> SMGGSPAGQKCFSRTVLAPGVVLIVQQGDLARLPVDVVVNASNEDLKHYGGLAAALSKAAGPELQADCDQIVKREGRLLPGNATISKAGK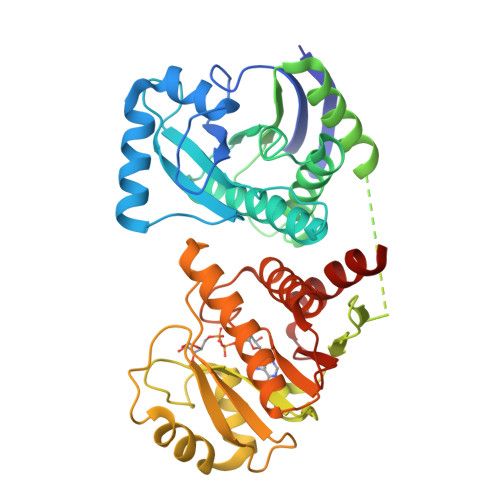LPYHHVIHAVGPRWSGYEAPRCVYLLRRAVQLSLCLAEKYKYRSIAIPAISSGVFGFPLGRCVETIVSAIKENFQFKKDGHCLKEIYLVDVSEKTVEAFAEAVKTVFKATLPDTAAPPGLPPAAAGPGKTSWEKGSLVSPGGLQMLLVKEGVQNAKTDVVVNSVPLDLVLSRGPLSKSLLEKAGPELQEELDTVGQGVAVSMGTVLKTSSWNLDCRYVLHVVAPEWRNGSTSSLKIMEDIIRECMEITESLSLKSIAFPAIGTGNLGFPKNIFAELIISEVFKFSSKNQLKTLQEVHFLLHPSDHENIQAFSDEFARRANGNLVS> SSQIRQNYSTEVEAA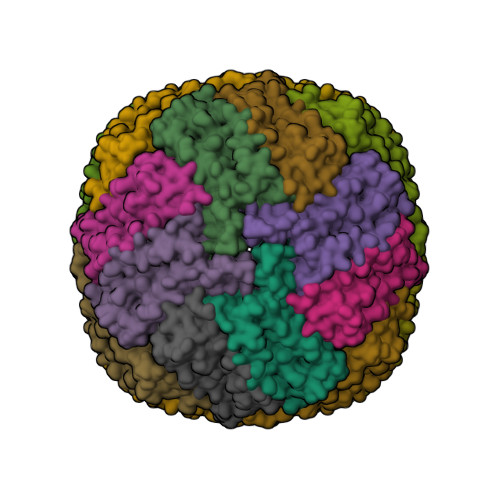VNRLVNLYLRASYTYLSLGFYFDRDDVALEGVCHFFRELAEEKREGAERLLKMQNQRGGRALFQDLQKPSQDEWGTTLDAMKAAIVLEKSLNQALLDLHALGSAQADPHLCDFLESHFLDEEVKLIKKMGDHLTNIQRLVGSQAGLGEYLFEHCTLKHD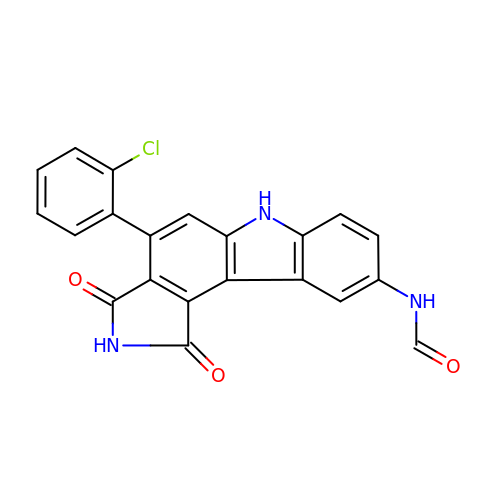N-[4-(2-CHLOROPHENYL)-1,3-DIOXO-1,2,3,6-TETRAHYDROPYRROLO[3,4-C]CARBAZOL-9-YL]FORMAMIDE | C21 H12 Cl N3 O3 | JWZVNUNTFNELHL-UHFFFAOYSA-N>MPAPEAPTSTLPPERPLTNLQQQIQQLVSRQPNLTAGLYFFNLDSGASLNVGGDQVFPAASTIKFPILVAFFKAVDEGRVTLQERLTMRPDLIAPEAGTLQYQKPNSQYAALEVAELMITISDNTATNMIIDRLGGAAELNQQFQEWGLENTVINNPLPDMKGTNTTSPR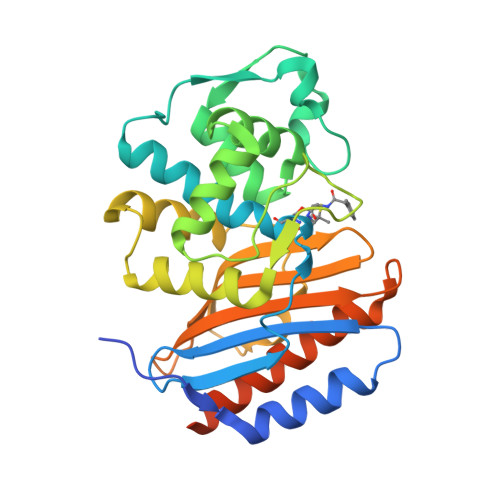DLATLMLKIGQGEILSPRSRDRLLDIMRRTVTNTLLPAGLGKGATIAHKTGDIGIVVGDAGMVDMPNGQRYVAAMMVKRPYNDPRGSELIRQVSRMVYQAFEKLSPPEQKLISEEDLNSAVDHHHHHH[4x]> FEDNF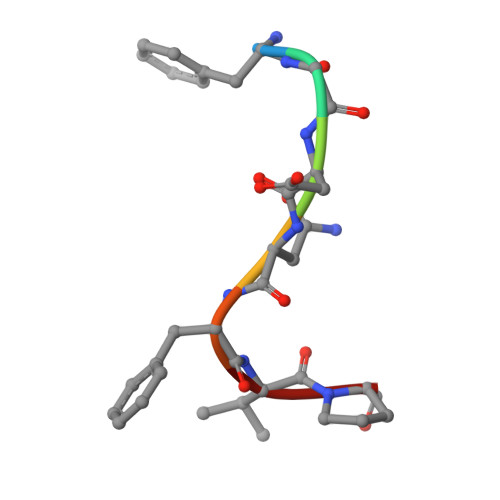VP>[2x]AQEEEAEQNLSELSGPWRTVYIGSTNPEKIQENGPFRTYFRELVFDDEKGTVDFYFSVKRDGKWKNVHVKATKQDDGTYVADYEGQN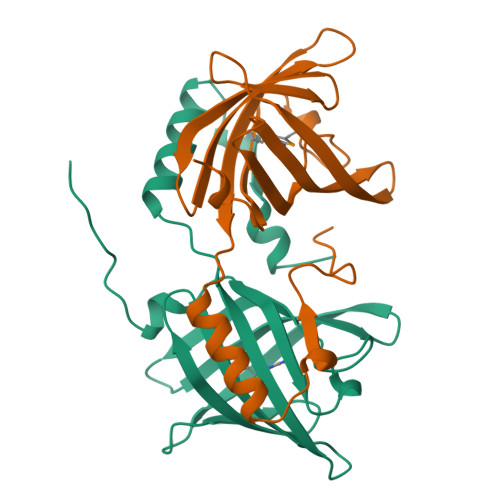VFKIVSLSRTHLVAHNINVDKHGQKTELTGLFVKLNVEDEDLEKFWKLTEDKGIDKKNVVNFLENEDHPHPE>[5x]ASQQFRIDSESIRDKLNTLLPSQSRGSIGVDLSGSTTIIPVVDLTETAEGGAQREDLQKAF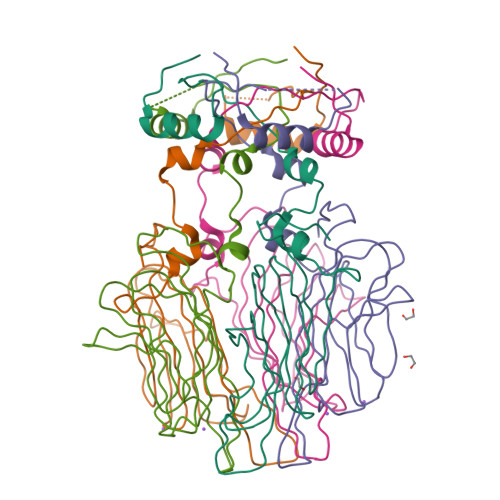TLINTIDFDVENTTTTIANTPGFYKVVGNLSSRDEASGAIAVIEVTDGITTKILANNRIVSPDGTTAVQSVPVPFDLMVKLVAGDTLQARSNNAEVRVQGIARQIADVSGNLINP(3P)-3-(4-chloro-2-ethoxyphenyl)-6-fluoro-2-[(piperazin-1-yl)methyl]quinazolin-4(3H)-one | C21 H22 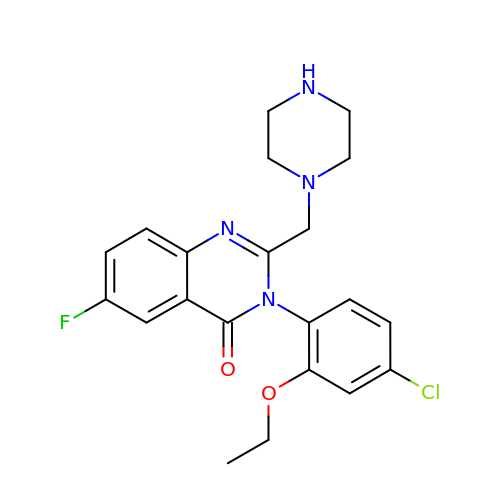Cl F N4 O2 | IKQWOCVGRWGJLP-UHFFFAOYSA-N> MLVCCRSSLSLLARATMPLCCSRRFLTHQNNIDDISGPVDTNSNSVSDGRLHCSTGEGGK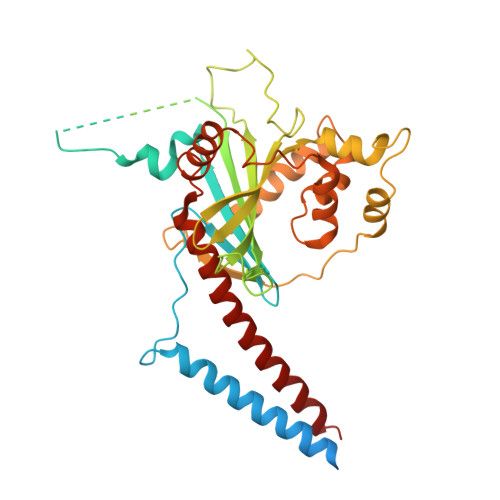ASTCERVSLRTIAESLGAAAAAELRAEVERDTRDGVAAIPPLPPLGWRVRHPSGSNYFVMTRTLKNGVQSAELNNRRYRSVHDIFLQSLQKGGHKYAQKGKGSEGRQKDAKEEEEPPSQEDGKSSPKVTVGYDREGRGHRATLQRMDELHDSPKLSRADVHLTVFAPFRVYDPSLHDPTVDICEWSSFDLVVQKTVPDNMVANKLLQPLSCTPQDGALSMYVCLASVNSEMRIRSIQLLSMKEAQALVEHACFGNGEPLFLELLRRRGRRRPLVERRFDDPRLRYEEVAQPQQVADEAAVACSSSCYGPYYPAFEMLMDSCGSAGEYSRALCYGGPYVSELSRELCDALLDYIKGDLGVSDQLCEYVCQMQFFLEQEEYMTWLGQVQHVANAVSRTA(9R,10E,12Z)-9-hydroxy-N-(2-hydroxyethyl)octadeca-10,12-dienamide 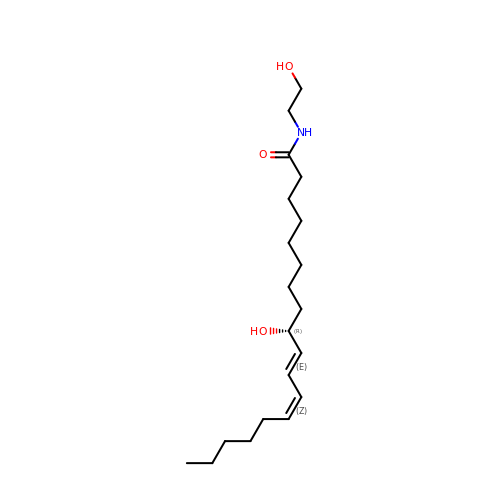| C20 H37 N O3 | VYCHZJQSKAOAAT-HGKNAVPSSA-N>MLSRKGIIPEEYVLTRLAEDPAEPRYRTRERRARFVSKKGNCNVAHKNIREQGRFLQDVFTTLVDLKWPHTLLIFTMSFLCSWLLFAMVWWLIAFAHGDLAPGEGTNVPCVTSIHSFSSAFLFSIEVQVTIGFGGRMVTEECPLAILILIVQNIVGLMINAIMLGCIFMKTAQAHRRAETLIFSKHAVITLRHGRLCFMLRVGDLRKSMIISATIHMQVVRKTTSPEGEVVPLHQVDIPMENGVGGNGIFLVAPLIIYHVIDSNSPLYDLAPSDLHHHQDLEIIVILEGVVETTGITTQARTSYLADEILWGQRFVPIVAEEDGRYSVDYSKFGNTIKVPTPLCTARQLDEDRSLLDALTLASSRGPLRKRSVAVAKAKPKFSISPDSLS[4x];>[4x]MPLAFCGTENHSAAYRVDQGVLNNGCFVDALNVVPHVFLLFITFPILFIGWGSQSSKVHIHHSTWLHFPGHNLRWILTFILLFVLVCEIAEGILSDGVT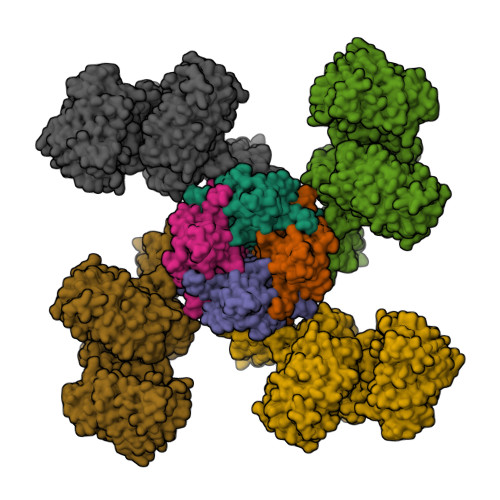ESRHLHLYMPAGMAFMAAITSVVYYHNIETSNFPKLLIALLIYWTLAFITKTIKFVKFYDHAIGFSQLRFCLTGLLVILYGMLLLVEVNVIRVRRYIFFKTPREVKPPEDLQDLGVRFLQPFVNLLSKGTYWWMNAFIKTAHKKPIDLRAIGKLPIAMRALTNYQRLCVAFDAQARKDTQSPQGARAIWRALCHAFGRRLILSSTFRILADLLGFAGPLCIFGIVDHLGKENHVFQPKTQFLGVYFVSSQEFLGNAYVLAVLLFLALLLQRTFLQASYYVAIETGINLRGAIQTKIYNKIMHLSTSNLSMGEMTAGQICNLVAIDTNQLMWFFFLCPNLWAMPVQIIVGVILLYYILGVSALIGAAVIILLAPVQYFVATKLSQAQRSTLEHSNERLKQTNEMLRGMKLLKLYAWESIFCSRVEVTRRKEMTSLRAFAVYTSISIFMNTAIPIAAVLITFVGHVSFFKESDLSPSVAFASLSLFHILVTPLFLLSSVVRSTVKALVSVQKLSEFLSSAEIREEQCAPREPAPQGQAGKYQAVPLKVVNRKRPAREEVRDLLGPLQRLAPSMDGDADNFCVQIIGGFFTWTPDGIPTLSNITIRIPRGQLTMIVGQVGCGKSSLLLATLGEMQKVSGAVFWNSNLPDSEGEDPSSPERETAAGSDIRSRGPVAYASQKPWLLNATVEENITFESPFNKQRYKMVIEACSLQPDIDILPHGDQTQIGERGINLSGGQRQRISVARALYQQTNVVFLDDPFSALDVHLSDHLMQAGILELLRDDKRTVVLVTHKLQYLPHADWIIAMKDGTIQREGTLKDFQRSECQLFEHWKTLMNRQDQELEKETVMERKASEPSQGLPRAMSSRDGLLLDEEEEEEEAAESEEDDNLSSVLHQRAKIPWRACTKYLSSAGILLLSLLVFSQLLKHMVLVAIDYWLAKWTDSALVLSPAARNCSLSQECDLDQSVYAMVFTLLCSLGIVLCLVTSVTVEWTGLKVAKRLHRSLLNRIILAPMRFFETTPLGSILNRFSSDCNTIDQHIPSTLECLSRSTLLCVSALTVISYVTPVFLVALLPLAVVCYFIQKYFRVASRDLQQLDDTTQLPLLSHFAETVEGLTTIRAFRYEARFQQKLLEYTDSNNIASLFLTAANRWLEVRMEYIGACVVLIAAATSISNSLHRELSAGLVGLGLTYALMVSNYLNWMVRNLADMEIQLGAVKRIHALLKTEAESYEGLLAPSLIPKNWPDQGKIQIQNLSVRYDSSLKPVLKHVNALISPGQKIGICGRTGSGKSSFSLAFFRMVDMFEGRIIIDGIDIAKLPLHTLRSRLSIILQDPVLFSGTIRFNLDPEKKCSDSTLWEALEIAQLKLVVKALPGGLDAIITEGGENFSQGQRQLFCLARAFVRKTSIFIMDEATASIDMATENILQKVVMTAFADRTVVTIAHRVHTILSADLVMVLKRGAILEFDKPETLLSQKDSVFASFVRADK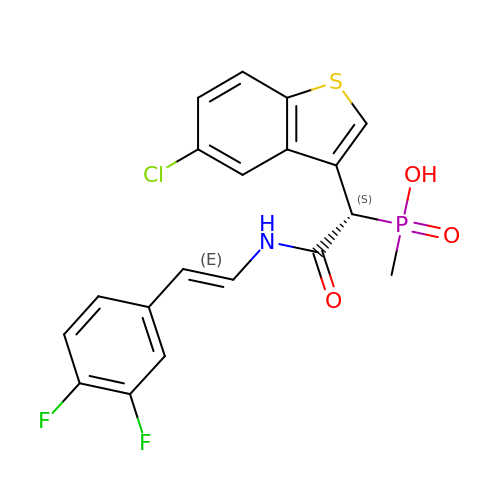(S)-[(1S)-1-(5-chloro-1-benzothiophen-3-yl)-2-{[(E)-2-(3,4-difluorophenyl)ethenyl]amino}-2-oxoethyl]methylphosphinic acid | C19 H15 Cl F2 N O3 P S | SEXLHAASDZPHOM-DKFQHHCZSA-N>MTGSNSHITILTLNINGLNSAIKRHRLASWIKSQDPSVCCIQETHLTCRDTHRLKIKGWRKIYQANGKQKKAGVAILVSDKTDFKPTKIKRDKEGHYIMVKGSIQQEELTILNIYAPNTGAPRFIKQVLSDLQRDLDSHTLIMGDFNTPLSTLDRSTRQKVN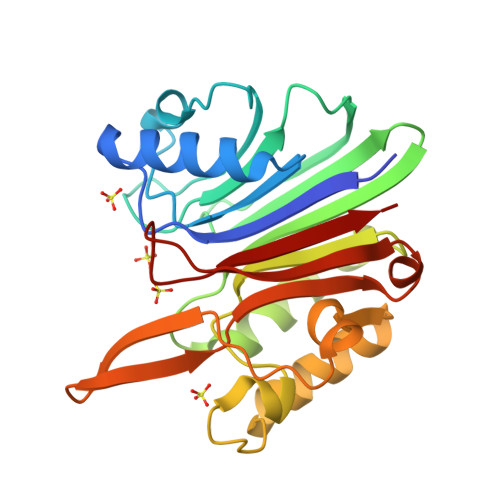KDTQELNSALHQADLIDIYRTLHPKSTEYTYVRVRDGHVSQSKIDHIVGSKALLSKCKRTEIITNYLSDHSAIKLELR[2x]Wnt proteins are a conserved family of secreted glycoproteins that govern essential developmental, growth, and regenerative processes and are also involved in pathological conditions such as cancer. We defined a signal peptide region in Wnts required for secretion on EVs, termed exosome-binding peptide (EBP). Coatomer was identified as the EV-binding protein for the EBP. Analysis of cocrystal structures, binding thermodynamics, and mutagenesis found that a dilysine motif mediates EBP binding to coatomer with a conserved function across the Wnt family.

Isothermal titration calorimetry (ITC) confirmed high affinity binding of the 18–amino acid EBP polypeptide with the N-terminal WD repeat of COPB2 with a dissociation constant (Kd) of 11.6 μM. The C-terminal half of the polypeptide (252 to 257) is bound to COPB2 with a Kd of 37.2 μM. To elucidate the molecular details for the interaction, we solved the structure of the EBP (252 to 257) bound to the COPB2 at 1.8-Å resolution by x-ray crystallography. The interaction involves two main contacts of the lysine side chains K253 and K255 with two acidic patches at the central opening of the β-propeller top face. More specifically, the amino groups of K253 and K255 interact with the carboxylate groups of D98 and D206 within the WD repeat domain (Saccharomyces cerevisiae COPB2 numbering). In addition to the two primary contacts, a secondary contact involves the backbone carbonyl oxygen atoms K255, K256, and P257 of EBP, which interact with the guanidinium groups of R59 and R101 and the amino group of K17 in the WD repeat domain. As expected, K255A or K253A substitutions markedly reduced or even abolished the EBP-COPB2 interaction, whereas K256A substitution, which is not involved in COPB2 binding, did not substantially affect the affinity. Immunoblot data corroborated that disruption of the KIK motif reduces the secretion of Wnt7a on EVs. COPB21–304 at 10 mg/ml (0.28 mM) was incubated with the Wnt252–257 peptide (LKIKKP) at 3 mM during 1 hour in 150 mM NaCl and 25 mM tris (pH 7.5) before setting the crystallization experiments. Best crystals were obtained in 0.1 M Hepes (pH 7.0) and 2.0 M AmSO4.

>MKLDIKKTFSNRSDRVKGIDFHPTEPWVLTTLYSGRVELWNYETQVEVRSIQVTETPVRAGKFIARKNWIIVGSDDFRIRVFNYNTGEKVVDFEAHPDYIRSIAVHPTKPYVLSGSDDLTVKLWNWENNWALEQTFEGHEHFVMCVAFNPKDPSTFASGCLDRTVKVWSLGQSTPNFTLTTGQERGVNYVDYYPLPDKPYMITASDDLTIKIWDYQTKSCVATLEGHMSNVSFAVFHPTLPIIISGSEDGTLKIWNSSTYKVEKTLNVGLERSWCIATHPTGRKNYIASGFDNGFTVLSLGNDE[24x];>LKIKKP[24x]>MNIHEWQSKQLIQKYGGRAQSGEVAFSPERSRDIAKKLWNQFPGCKFVVKAQVLAGGRGKGHWEHGMQGGVKLAKTPEEVYEIANEMIGHKLITKQTGAKGINCNKVMVCGAVKILKEFYLSILLDRAMGCPVIIA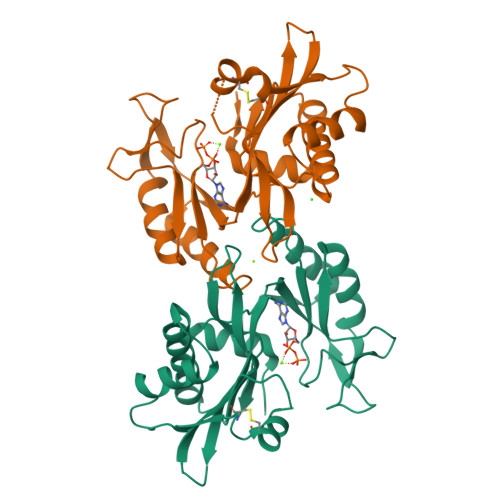TSQGGMGIEEVAQKCPECLFKVPISVKNGPTNEQLVKLAKDLGLEGDLVQDCVDNVKALYQVFDKCDSTMVEINPLGVIETPTDEKVICCLDAKIAFDKDAAFGLEHHHHHHHH[2x]> PHMSGLKKFFPYSTNVLKGAAADIALPSLAGKTVFFYFSASWCPPCRAFTPQLIDFYKAHAESKNFEVMLISWDESAEDFKDYYA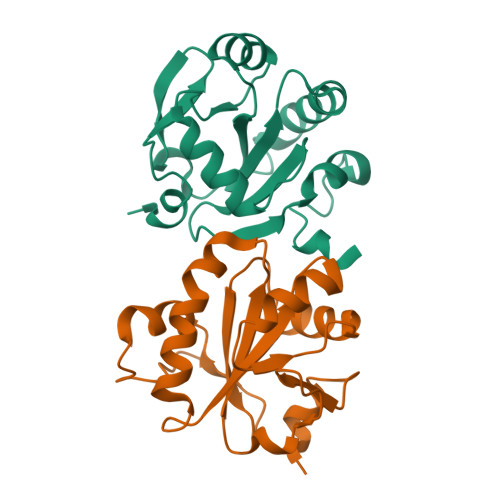KMPWLALPFEDRKGMEFLTTGFDVKSIPTLVGVEADSGNIITTQARTMVVKDPEAKDFPWPNVEAKK;> PHMSGLKKFFPYSTNVLKGAAADIALPSLAGKTVFFYFSASWCPPCRAFTPQLIDFYKAHAEKKNFEVMLISWDESAEDFKDYYAKMPWLALPFEDRKGMEFLTTGFDVKSIPTLVGVEADSGNIITTQARTMVVKDPEAKDFPWPNVEAKK>[16x]MCFSPKISTPKPSVQAPEPAPLSEEVASVDIGAESDVDTNETKGIKDLKVKKESAPKDKSSVSRAMRNSGVNMG;>MASNIESALANRTMGRGRAPGKTIAVNYQAASVQAPTGDSGLARALTSFVESGTGL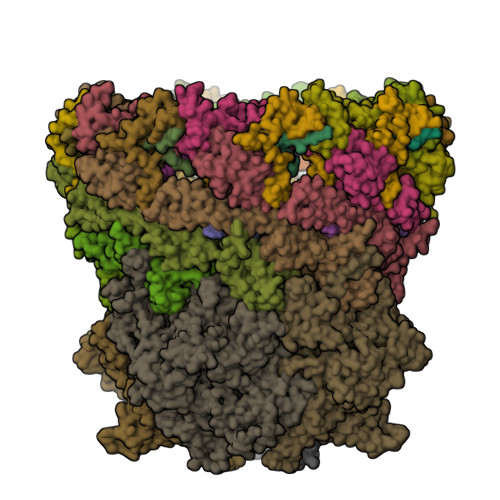YKQFKDEEKTRADERSNEIIRKLTPQQRREAIQNGTLLYQDDPYAMEALRVKTGRNAAFAVDDEINVKIQNGEFRTRQDMEEYRHQRLQDAAKSYAEEAGINPTDEFFQRGFNDNITDRNIAIYGSFNKYFSKQSEETAMLNTRIEMNSFLNDGDLMRSPESGKTFMAYLRDGLTTAAIPSDQRAREVITQTVRDAIQKSGGSNFLQQVRGERITLNGVDATVEEIVGPDVFNAAIVEAQGTEYKLVAKYQEDLALGVQSAILQDDPTIGLAQIQKLKEQNNLLQPGEELTPQRQMLINAEASLLEAVKRKSAEQAKENTKLIQTQNKQLVIDQVYQRRLAGDNVSTNYEDLPVSEATGEFKRSDMNNYASAKLQQIDQMDIPEAAKDAQKVALLRADTNNGPFRNAFQTLTQDAAGEWQAAVIRGQYDPDKMQRFESLRRAYTQDPSSFAALYPDQAQLFSTFDQMDKIGLDPQTMIEADKQAASQSREMRMESDKAWQELKNDSRNKDLSRLPTSLDASARKVWDSWYYRTGNADAATQQTQRWLNENTVTFQSEGSDGKSIGMVSKHQLMVGDNPESWQVGRDIIDTARKQLIKANPWVVNSQLSVVEQNGSIFLQDATGTIRIRYDKELVGKLYREQQQKAQDAAYAQAERDANKRARIVGTKAAGDKRRADREANIEKRGGMYNDVSLEGIAKVLIGKE[8x];>MCEPVSIGLGIMSVAGATMSASQQAKAEGAAIDAQNRQAQEMIKQMNYSDANLKMQERDLKEQQMAELTETTLNGIRNQGMVRAAVAESGLEGNSMDRIERQVAGDTVKERAGITESYNRDYAAIFGNRIANIENTQSAIRGQGKIIKTSPLAHALNVATAGVQGYAAGKSMSGTSGSGGAAPISAAKGTPTGHS[8x];>[4x]MATRGIRNNNPGNIRVSKDQWEGMTGDDGAFVTFDSPESGVRALGKNLLSYGRQGYDSIEKIINRWAPPNENDTKAYIDSVVAATGIPATQSLDLSNQDTLSALAQAISFHETGSRYDPEVYQKGVARALNGISPKTPPVSANVFDALTEGLKAKPKVALGENLPTAAGLNIEGQAPEAPNESFGEMFYKSTGETMQEREDRSTWFGFGAATEAEVKNSMVGVAIRAGQTEDSLDVIGDVFNPTRWNNHKWTREELDQIRNAGVLPQYYGVITGGSPQNLTELINLALENQKLDQEKAKAGTGAQLAAGVIGAGVDPLTYVPIAGQVGKGGKLVNKMFTVAAQSGALAGVSEMARTSVAGGDAHVAEAILGGALFGGGMTAIADGLGRALGRNTNEFAGPATRLEARETARNVDGQDLSRLPIQEGEQTFSHQGVKFADVPNEPGSVRLEDGSILIGENPLNPKTRQVFDEVIEPERAAAGVNLGGLTEIGLKLLRSENPEIRGVAADLVRSPTGMQSGASGKIGTTASDVFERLRAVDHRFYNDIDDAVTEALKDPYFQTAFWRDSGAFRQDIYQRVSMAIEDGSGNLKAELTPGELKVYDLLKNQFDAKREMMENPAMFGRPDAQSIFPGSRFKGTYVPHVYSSQMKELYIKELGSPEALQEAIKKSWLTSYASRPEVKKRVDEALLEADPTLTPEGLAAAVDKYANDKAYGISHTEQFERSSVMEENINGLVGLENNSFLEARNLFDSDMSIVLPNGQTFSVNNLREWDMDKIVPAYNRRVNGDIAIMAGTGKTTKEMKDLVETLMNKAGDDGKLKGEVSTLRDTLKILTGRARRDGADDAAFATVMRTMTDLAFFAKNAYMGVQNLTEIGGMLARGNVRAMLHGVPMFRDLAFRNKKVGASEIKDLHNVIFGKELDDSIRPSKQDVIDRLRSYSDLGRGAATALGTAKYYTGELAVRSPFTKVLNGTTNYLLDAGRQGFLSDIVEHSLTGSKRRFDDRWLKTAGISDEQWKGIKSLIRESVTRGPDGKYTIKDKKAFSQDQRAMDLWRMGDTIADETLLRPHKLSNMDAKAYGPIAKTVLQFKNFVIKSINGRTMRTFYNATKNNRAMDAALSTVMSMGLAGMYYMAQAHIKAYAMQDGRDREYLKQALNPTMIGYAALSRSSHLGGPLGVANILGGIAGYEDTKMLRSSILPRSPTEKTEKPIAFGAASSGPVMNVVGNFLEQVPAFGYAANVGATAYNLAGYLKADTRVNERDYMTGMYNTFRELVPNDPITQKLLLGTFEEQGIHIKD>MDILLVDGYNMIGAWPQLKDLKANSFEEARDVLIQKMAEYQSYTGNRVIVVFDAHLVKGLEKKQTNHRVEVIFTKENETADERIEKLAQALNNIATQIHVATSDYTEQWAIFGQGALRKSARELLREVET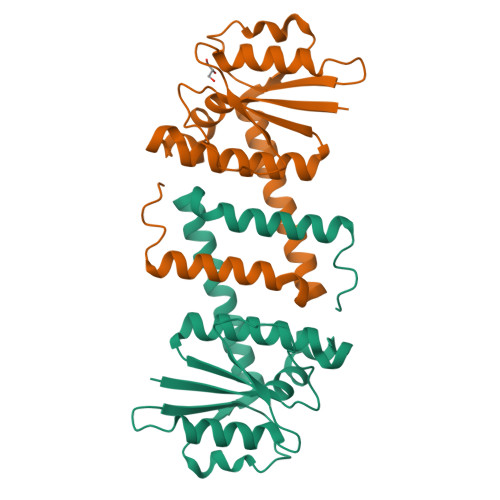IERRIERRVRKITSEKPAGKIALSEEVLKTFEKWRRGDLDAAALEHHHHHH[2x]> MAYRKRGARREANINNNDRMQEKDDEKQDQNNRMQLSDKVLSKKEEVVTDSQEEIKIADEVKKSTKEESKQLLEVLKTKEEHQKEIQYEILQKTIPTFEPKESILKKLEDIKPEQAKKQTKLFRIFEPRQLPIYRANGEKELRNRWYWKLKKDTLPDGDYDVREYFLNLYDQVLTEMPDYLLLKDMAVENKNSRDAGKVVDSETASICDAIFQDEETEGAVRRFIAEMRQRVQADRNVVNYPSILHPIDYAFNEYFLQHQLVEPLNNDIIFNYIPERIRNDVNYILNMDRNLPST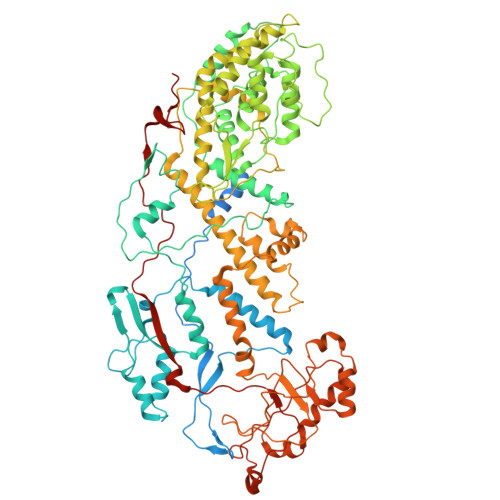ARYIRPNLLQDRLNLHDNFESLWDTITTSNYILARSVVPDLKELVSTEAQIQKMSQDLQLEALTIQSETQFLTGINSQAANDCFKTLIAAMLSQRTMSLDFVTTNYMSLISGMWLLTVVPNDMFIRESLVACQLAIVNTIIYPAFGMQRMHYRNGDPQTPFQIAEQQIQNFQVANWLHFVNNNQFRQVVIDGVLNQVLNDNIRNGHVINQLMEALMQLSRQQFPTMPVDYKRSIQRGILLLSNRLGQLVDLTRLLAYNYETLMACVTMNMQHVQTLTTEKLQLTSVTSLCMLIGNATVIPSPQTLFHYYNVNVNFHSNYNERINDAVAIITAANRLNLYQKKMKAIVEDFLKRLHIFDVARVPDDQMYRLRDRLRLLPVEVRRLDIFNLILMNMDQIERASDKIAQGVIIAYRDMQLERDEMYGYVNIARNLDGFQQINLEELMRTGDYAQITNMLLNNQPVALVGALPFVTDSSVISLIAKLDATVFAQIVKLRKVDTLKPILYKINSDSNDFYLVANYDWVPTSTTKVYKQVPQQFDFRNSMHMLTSNLTFTVYSDLLAFVSADTVEPINAVAFDNMRIMNEL> VTAASGFVDLATFSDLEAYLYGGCSAVTYFVRAIKKANWFSFLPVVLRNISGLPGFGSEFSASVNRSGDYVLNTWLRVRLPLVAIRPTNTGGAINANATIRWTRNFMHNLVEKVNITFNDLIVHEFDSYWFDFNSQFNIDASKRVGYRNMIGDIPAMINPVTTGNPLGTGEFFNLPIPLFYTEDSGLALAVSALPFNDIKINYCLRRWQDLIVLNVGVGGNPPTYDDIVQVSYDSTFTLIYSSNAPAITNVETWCHYAVVHNDERVKMGKNPRDMVIKQVQKVNETTINLSQLNALVPIDIRVSHAVVGYFYAIRNSSTTGEWSNYTTEPAYAGLDPLEAAQLVYESTARVSNGSDYYSLMVPWYWHKSIPEETGYHAYSYSLDTFASDPKGSTNYSKLTNVSNQYV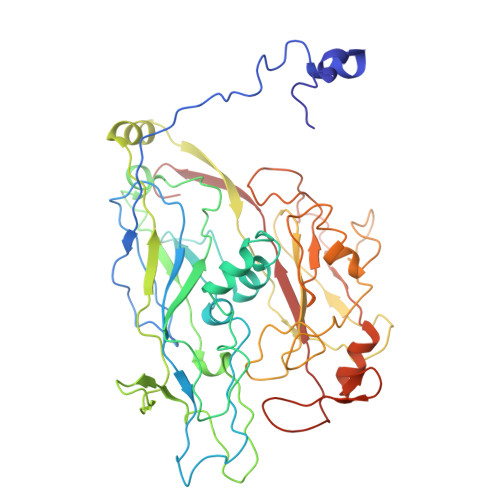PSTAAVNASAGVTNTGIPIPSATNPAVTQQNQTFQHIFRVLNFNVLRLSGGS> MEACPHIRYAFQNDKLLLQQASVGRLTLVNKTTILLRPMKTTTVDLGLYARPPEGHGLMLWGSTSRPVTSHVGIIDPGYTGELRLILQNQRRYNSTLRPSELKIHLAAFRY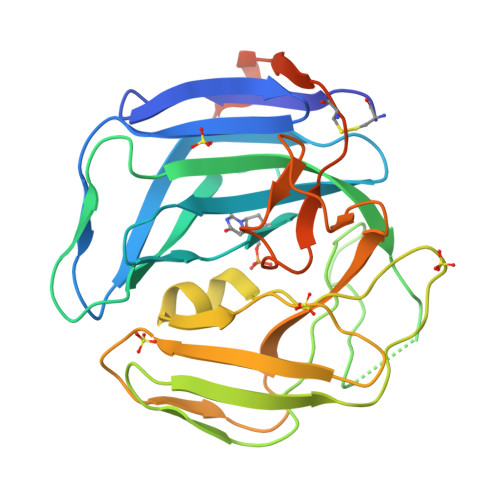ATPQMEEDKGPINHPQYPGDVGLDVSLPKDLALFPHQTVSVTLTVPPPSIPHHRPTIFGRSGLAMQGILVKPCRWRRGGVDVSLTNFSDQTVFLNKYRRFCQLVYLHKHHLTSFYSPHSDAGVLGPRSLFRWASCTFEEVPSLAMGDSGLSEALEGRQGRGFGSSGQ>[2x]MAKLTRLGDLERAVMDHLWSRTEPQTVRQVHEALSARRDLAYTTVMAVLQRLAKKNLVLQIRDDRAHRYAPVHGRDELVAGLMVDALAQAEDSGSRQAALVHFVERVGADE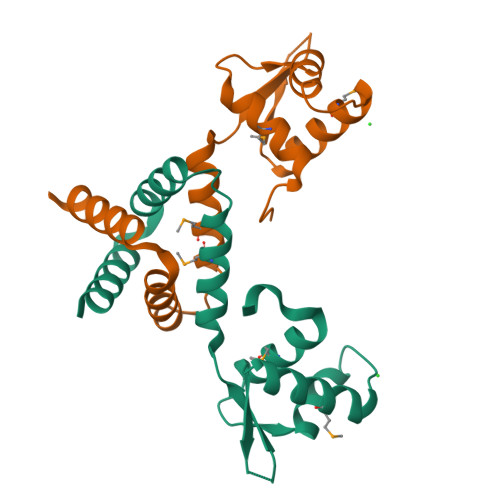ADALRRALAELEAGHGNRPPAGAATET> LPRVKHTLVPPPFAHAHEQVAASGPVINEFEMRIIEKEVQLDEDAYLQAMTFDGSIPGPLMIVHEGDYVELTLINPPENTMPHNIDFHAATGALGGGGLTLINPGEKVVLRFKATRAGAFVYHCAPGGPMIPWHVVSGMAGCIMVLPRDGLKDHEGKPVRYDTVYYIGESDHYIPKDEDGTYMRFSDPSEGYEDMVAVMDTLIPSHIVFNGAVGALTGEGA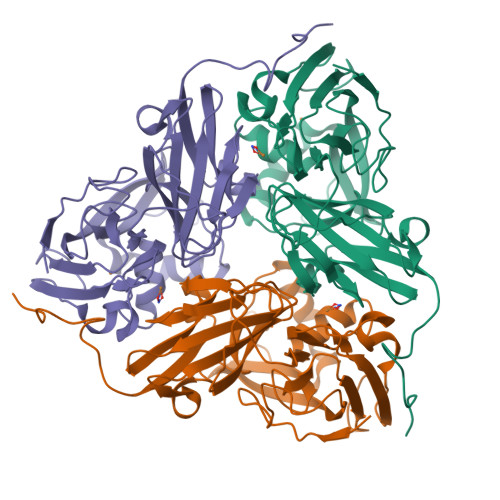LKAKVGDNVLFVHSQPNRDSRPHLIGGHGDLVWETGKFHNAPERDLETWFIRGGSAGAALYKFLQPGVYAYVNHNLIEAVHKGATAHVLVEGEWDNDLMEQVVAPVG ATP-sensitive potassium channels (KATP), composed of Kir6 and SUR subunits, convert the metabolic status of the cell into electrical signals. Functional KATP channels are hetero-octamers composed of four Kir6 subunits and four SUR subunits. SUR subunits are not only targeted by inhibitors, such as insulin secretagogues, but also by activators, such as KATP openers. Here, we present cryo-EM structures of SUR2A and SUR2B subunits in complex with Mg-nucleotides and P1075 or levcromakalim, two chemically distinct KATP openers that are specific to SUR2.

To understand how KATP openers are engaged with SUR2, we further solved the structure of SUR2B in complex with P1075, SUR2B in complex with Lev, and SUR2A in complex with P1075 to the resolutions of 3.3 Å, 3.1 Å, and 3.3 Å, respectively. Additionally, SUR2 has two splicing isoforms, namely SUR2A and SUR2B, which differ in their C-terminal 42 residues. P1075 robustly activates both SUR2A and SUR2B28. The cryo-EM maps of P1075 in complex with both SUR2A and SUR2B show that P1075 sits in the middle of SUR2 TMD and is embraced by TM10, TM11, TM12, TM14, and TM17 helices. We named this pocket the “KATP channel opener-binding site” (KCOS). The C-terminal 42 residues of SUR2 fold into α7 to α9, which is part of NBD2. Although these residues are different between SUR2A and SUR2B, we found that their structures are highly similar in the Mg-ADP/Mg-ATP and P1075-bound states with an RMSD of 0.327 Å. Although SUR2A and SUR2B differ in Mg-ADP activation and KATP opener sensitivity, their structures are highly similar in the Mg-nucleotides and KATP opener-bound state. Therefore, we speculate the structures of SUR2A and SUR2B might have structural variations in the NBD-separated inward-facing conformation and such structural difference leads to the functional differences between SUR2A and SUR2B. Although we prepared the SUR2B + P1075 samples using Mg-ATP alone, while other SUR2 samples using both Mg-ADP and Mg-ATP, we found that Mg-ATP was bound in the degenerate site and Mg-ADP was bound in the consensus site in all of the structures.

> MSLSFCGNNISSYNIYHGVLQNPCFVDALNLVPHVFLLFITFPILFIGWGSQSSKVQIHHNTWLHFPGHNLRWILTFALLFVHVCEIAEGIVSDSQRASRHLHLFMPAVMGFVATTTSIVYYHNIETSNFPKLLLALFLYWVMAFITKTIKLVKYWQLGWGMSDLRFCITGVMVILNGLLMAVEINVIRVRRYVFFMNPQKVKPPEDLQDLGVRFLQPFVNLLSKATYWWMNTLIISAHRKPIDLKAIGKLPIAMRAVTNYVCLKEAYEEQKKKAADHPNRTPSIWLAMYRAFGRPILLSSTFRYLADLLGFAGPLCISGIVQRVNEPKNNTTRFSETLSSKEFLENAHVLAVLLFLALILQRTFLQASYYVTIETGINLRGALLAMIYNKILRLSTSNLSMGEMTLGQINNLVAIETNQLMWFLFLCPNLWAMPVQIIMGVILLYNLLGSSALVGAAVIVLLAPIQYFIATKLAEAQKSTLDYSTERLKKTNEILKGIKLLKLYAWEHIFCKSVEETRMKELSSLKTFALYTSLSIFMNAAIPIAAVLATFVTHAYASGNNLKPAEAFASLSLFHILVTPLFLLSTVVRFAVKAIISVQKLNEFLLSDEIGEDSWRTGEGTLPFESCKKHTGVQSKPINRKQPGRYHLDNYEQARRLRPAETEDVAIKVTNGYFSWGSGLATLSNIDIRIPTGQLTMIVGQVGCGKSSLLLAILGEMQTLEGKVYWNNVNESEPSFEATRSRSRYSVAYAAQKPWLLNATVEENITFGSSFNRQRYKAVTDACSLQPDIDLLPFGDQTEIGERGINLSGGQRQRICVARALYQNTNIVFLDDPFSALDIHLSDHLMQEGILKFLQDDKRTVVLVTHKLQYLTHADWIIAMKDGSVLREGTLKDIQTKDVELYEHWKTLMNRQDQELEKDMEADQTTLERKTLRRAMYSREAKAQMEDEDEEEEEEEDEDDNMSTVMRLRTKMPWKTCWWYLTSGGFFLLFLMIFSKLLKHSVIVAIDYWLATWTSEYSINDPGKADQTFYVAGFSILCGAGIFLCLVTSLTVEWMGLTAAKNLHHNLLNKIILGPIRFFDTTPLGLILNRFSADTNIIDQHIPPTLESLTRSTLLCLSAIGMISYATPVFLIALAPLGVAFYFIQKYFRVASKDLQELDDSTQLPLLCHFSETAEGLTTIRAFRHETRFKQRMLELTDTNNIAYLFLSAANRWLEVRTDYLGACIVLTASIASISGSSNSGLVGLGLLYALTITNYLNWVVRNLADLEVQMGAVKKVNSFLTMESENYEGTMDPSQVPEHWPQEGEIKIHDLCVRYENNLKPVLKHVKAYIKPGQKVGICGRTGSGKSSLSLAFFRMVDIFDGKIVIDGIDISKLPLHTLRSRLSIILQDPILFSGSIRFNLDPECKCTDDRLWEALEIAQLKNMVKSLPGGLDATVTEGGENFSVGQRQLFCLARAFVRKSSILIMDEATASIDMATENILQKVVMTAFADRTVVTIAHRVSSIMDAGLVLVFSEGILVECDTGPNLLQHKNGLFSTLVMTNK>[2x]MKSADQLMSDIQLSLQALFQKIQPEMLESMEKQGVTPAQLFVLASLKKHGSLKVSEIAERMEV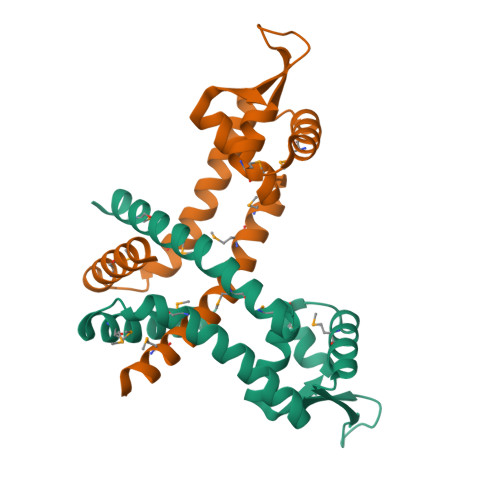KPSAVTLMADRLEQKNLIARTHNTKDRRVIDLSLTDEGDIKFEEVLAGRKAIMARYLSFLTEEEMLQAAHITAKLAQAAETDEKQNMKRGNG>MAVTYEKTFEIEIINELSASVYNRVLNYVLNHELNKNDSQLLEVNLLNQLKLAKRVNLFDYSLEELQAVHEYWRSMNRYSKQVLNKEKVA[2x];>MANIVNFTDKQFENRLNDNLEELIQGKKAVESPTAFLLGGQPGSGKTSLRSAIFEETQGNVIVIDNDTFKQQHPNFDELVKLYEKDVVKHVTPYSNRMTEAIISRLSDQGYNLVIEGTGRTTDVPIQTATMLQAKGYETKMYVMAVPKINSYLGTIERYETMYADDPMTARATPKQAHDI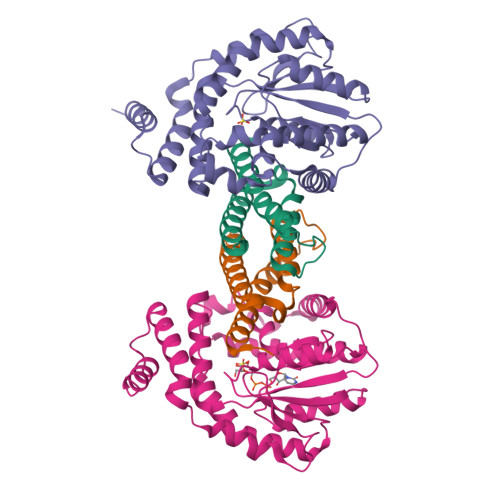VVKNLPTNLETLHKTGLFSDIRLYNREGVKLYSSLETPSISPKETLEKELNRKVSGKEIQPTLERIEQKMVLNKHQETPEFKAIQQKLESLQPPTPPIPKTPKLPGI[2x]>[3x]MKVLFLTANEFEDVELIYPYHRLKEEGHAVYIASFERGTITGKHGYSVKVDLTFDKVNPAEFDALVLPGGRAPERVRLNAKAVSIARKMFSEGKPVASICHGPQILISAGVLRGRKGTSYPGIKDDMINAGVEWVDAEVVVDGNWVSSRVPADLYAWMREFVKLLK

Here, a microfluidic device is described that enables the production of crystals by counter-diffusion and their direct on-chip analysis by serial crystallography at room temperature. Furthermore, the crystal structures of four proteins and an RNA were determined based on serial data collected on four synchrotron beamlines, demonstrating the general applicability of this multipurpose chip concept.

Tb-Xo4 was added to the protein solution before filling the channels. It triggered the nucleation and the growth of large PhP1 crystals, which completely filled the available volume. An added value for macromolecules crystallized in the presence of Xo4 is the strong luminescence when illuminated by UV light. Final crystal structures were obtained either from a single large crystal and two wedges (Nb02) or from combining partial data sets from several individual crystals (RNA, CCA, Lip and PhP1). In the latter case, the use of ccCluster considerably facilitated the choice of partial data sets to be merged.> MTLESALTLFVAVPLLTAGVLVAVASRTRLILTVLFAVLGTQLAAAVATVPWVSDGSVVVHQVALWAPGVSIPFVLDMFSALMLTVTSLLTLTCAAFAVAAGEAYKRFYPPLVLLVTAGVNGALLTGDLFNFFVFVEVMLLPSYGLMMITRSGRASVVGVAASRLYISVNLLASTILLIGVALIYGVTGTVNIAQLHGAASEDTAVAVATALVLFALAIKAAVVPVHGWLARAYPKMSPAVTAMFSGLHTKIAIYAIYRIYAVIFDGDSRYLWVGVVVFSATMLIGVLGAVGEAAPRSILAFHMVSQIGYILLGVALFGPIGLTAGIFYLLHHMIVKAALFLAIGAIEVRYGPRRLGQLSGLAKTEPLVAVAFFASAMSLAGIPPFSGFVAKLSLIIAALDAGQIAAAAVAVVVSILTLLSMLKIWTGIFLGEPTPTDSRTLPEGLDPAHSEATGI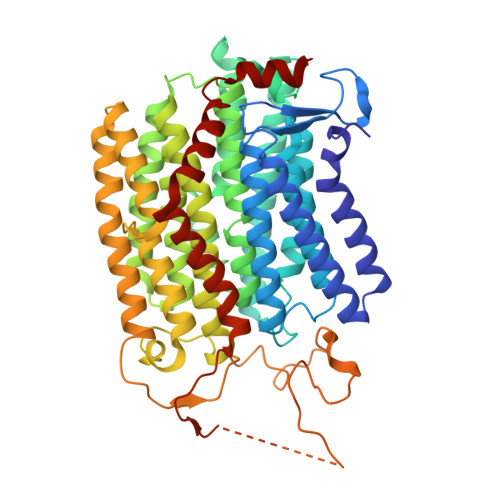PDGRDVDGRHRDGVEITGAAAGATPTDTMAPASTTATATATDTVTETASVADTAEAGSPDPDMVPPGRRIGLALAAPALALSVVTLALGLGGQLLLELSGTAAANLYDPTTYIQAVLG Analogous to ubiquitination, ufmylation is carried out by a three-enzyme cascade involving E1, E2, and E3 proteins. The E1 UBA5 has three distinct regions: (1) an adenylation domain that binds ATP and magnesium ions; (2) a UFM1-interacting sequence (UIS) spanning amino acids 334 to 346 that holds UFM1 in a trans binding mechanism; and (3) a UFC1-binding sequence (UBS) from 392 to 404 that binds UFC117–21. The adenylated UFM1 is then subjected to a nucleophilic attack by the catalytic C250 of UBA5 to form a thioester bond with the C-terminal glycine of UFM1. This is followed by a trans thiolation process, whereby the UFM1 is transferred to the E2 UFC1 forming a thioester bond with C116 of UFC1. However, UBA5 does not harbor such a domain but instead has a short sequence called UBS that is responsible for the interaction with UFC128.

Therefore, to gain structural insights about this region and how it interacts with UFC1, we attempted to crystalize UFC1 in complex with UBA5 347–404, but with no success. However, we successfully crystallized and determined the structure of UBA5(347–404) that is fused to the N-terminus of UFC1 to 2.65 Å resolution. The asymmetric unit contains one fusion molecule, and UFC1 interacts with the UBS that arrives from another asymmetric unit. As expected, the interaction of the UBS with UFC1 retains the same architecture as observed in the structure with the shorter fragment containing only the UBS sequence. In both structures, the UBS binds to the α-1 helix and β-1 strand of UFC1. However, for the linker connecting the UBS, we obtained electron density for residues 382–389 but not for 347–381, suggesting that most of the linker is mobile. V382 (the first built residue at the N-terminus of UBA5) is 35 Å away from UFC1 C116. While this distance is far from the active site, UBA5 residues 381–363 can span it, thereby we cannot rule out the possibility that the linker reaches the vicinity of UFC1 active site Cys.

> GSEVSEEELKNFSGPVPDLPEGITVAYTIPKKQEDSVTELTVEDSGESLEDLMAKMKNMMADEATRRVVSEIPVLKTNAGPRDRELWVQRLKEEYQSLIRYVENNKNADNDWFRLESNKEGTRWFGKCWYIHDLLKYEFDIEFDIPITYPTTAPEIAVPELDGKTAKMYRGGKICLTDHFKPLWARNVPKFGLAHLMALGLGPWLAVEIPDLIQKGVIQHKEKCNQ> SMGLFAKQVQKK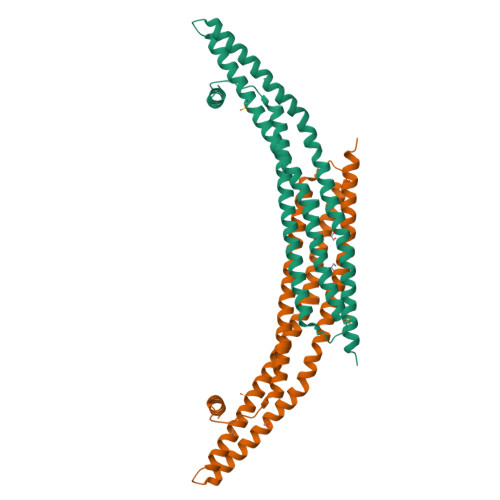FSRAQEKVLQKLGKAVETKDERFEQSASNFYQQQAEGHKLYKDLKNFLSAVKVMHESSKRVSETLQEIYSSEWDGHEELKAIVWNNDLLWEDYEEKLADQAVRTMEIYVAQFSEIKERIAKRGRKLVDYDSARHHLEAVQNAKKKDEAKTAKAEEEFNKAQTVFEDLNQELLEELPILYNSRIGCYVTIFQNISNLRDVFYREMSKLNHNLYEVMSKLERQHSNK N-hydroxypropanamide 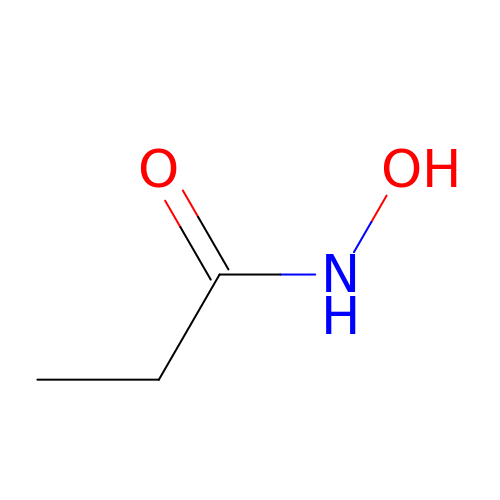| C3 H7 N O2 | RSIPQHOWTCNEBI-UHFFFAOYSA-N>[8x]MAAAAGRSLLLLLSSRGGGGGGAGGCGALTAGCFPGLGVSRHRQQQHHRTVHQRIASWQNLGAVYCSTVVPSDDVTVVYQNGLPVISVRLPSRRERCQFTLKPISDSVGVFLRQLQEEDRGIDRVAIYSPDGVRVAASTGIDLLLLDDFKLVINDLTYHVRPPKRDLL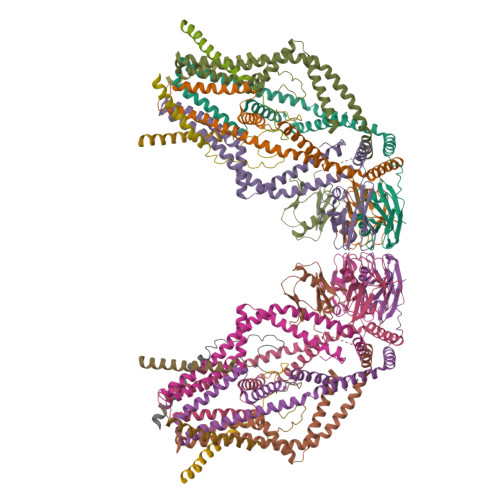SHENAATLNDVKTLVQQLYTTLCIEQHQLNKERELIERLEDLKEQLAPLEKVRIEISRKAEKRTTLVLWGGLAYMATQFGILARLTWWEYSWDIMEPVTYFITYGSAMAMYAYFVMTRQEYVYPEARDRQYLLFFHKGAKKSRFDLEKYNQLKDAIAQAEMDLKRLRDPLQVHLPLRQIGEKD;>[8x]MASGAARWLVLAPVRSGALRSGPSLRKDGDVSAAWSGSGRSLVPSRSVIVTRSGAILPKPVKMSFGLLRVFSIVIPFLYVGTLISKNFAALLEEHDIFVPEDDDDDD>[4x]SNAMDKIVVQGGDNRLVGSVTIEGAKNAVLPLLAATILASEGKTVLQNVPILSDVFIMNQV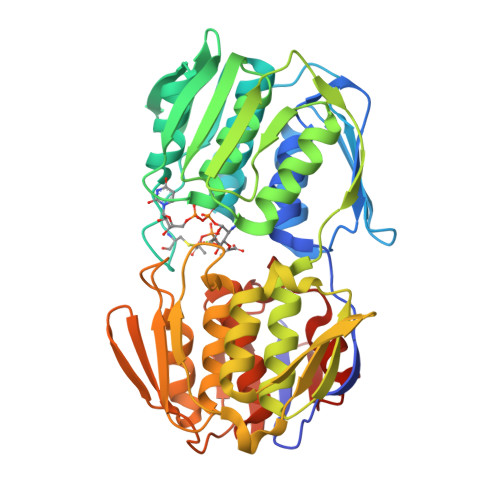VGGLNAKVDFDEEAHLVKVDATGDITEEAPYKYVSKMRASIVVLGPILARVGHAKVSMPGGCTIGSRPIDLHLKGLEAMGVKISQTAGYIEAKAERLHGAHIYMDFPSVGATQNLMMAATLADGVTVIENAAREPEIVDLAILLNEMGAKVKGAGTETITITGVEKLHGTTHNVVQDRIEAGTFMVAAAMTGGDVLIRDAVWEHNRPLIAKLLEMGVEVIEEDEGIRVRSQLENLKAVHVKTLPHPGFPTDMQAQFTALMTVAKGESTMVETVFENRFQHLEEMRRMGLHSEIIRDTARIVGGQPLQGAEVLSTDLRASAALILTGLVAQGETVVGKLVHLDRGYYGFHEKLAQLGAKIQRIEASDEDE> AGCGGGGU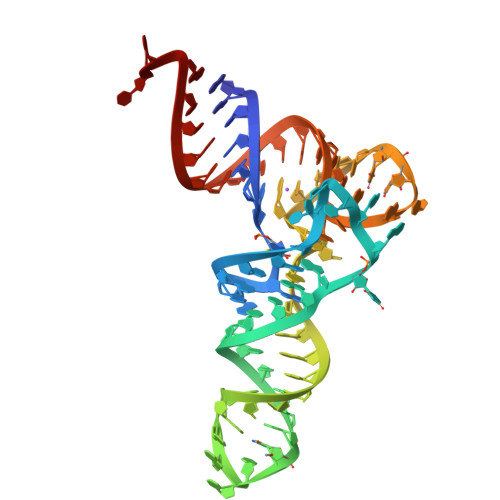GGAGCAGCCUGGUAGCUCGUCGGGCUCAUAACCCGAAGAUCGUCGGUUCAAAUCCGGCCCCCGCUACCA The A2HBD has elevated expression in F. prausnitzii A2-165 and is crucial for the transformation of acetoacetyl-CoA to 3-hydroxybutyryl-CoA in the butyrate cycle. The monomeric structure of A2HBD consists of two domains, N-terminal and C-terminal, with cofactor binding occurring at the N-terminal domain, while the C-terminal domain facilitates dimerization. The A2HBD protein exists as a hexamer in solution.

To ascertain the binding mode of NAD+, we determined the 2.55Å resolution crystal structure of A2HBD in complex with NAD+ cofactor. In the structural analysis of the NAD+ complex derived from crystallography within the P21 space group, it was observed that all subunits comprising the hexameric assembly were found to bind to NAD+. By superposing the NAD-bound form of A2HBD with the apo-enzyme, we observed that the monomer structure of the NAD complex is similar to the apo-enzyme structure, displaying a root-mean-square deviation of 0.543Å. Like other NAD-dependent dehydrogenase enzymes, the NAD+ cofactor binds to the Rossmann fold domain without forming significant interactions with the C-terminal domain. Observing the binding mode of the NAD cofactor, adenine moiety of NAD cofactor is somewhat exposed to the surface of the enzyme, and the ribose and nicotinamide portion fitted into the deep cleft facing the acetyl group of the substrate. The phosphate moiety of the NAD cofactor resides within the G-x-G-x-x-G motif, composed of Gly7-Ala8-Gly9-Thr10-Met11-Gly12, situated between the initial β strand and the first α a helix within the Rossmann fold domain. The NAD cofactor is captured by the enzyme’s Thr10 and Met11 main-chain nitrogen atoms, establishing hydrogen bonds with the hydroxyl group of the phosphate moiety. Hydrogen bonding interactions involving Asp31, Glu90, Lys95, Asn115, and Ser117, along with hydrophobic interactions with Met11 and Phe138, contribute to the stabilization of the NAD cofactor’s two ribose rings and nicotinamide moiety. The hydrophobic pit accommodates the adenine moiety, fostering interactions with hydrophobic residues such as Ile6, Ile32, Ala88, Phe,89, Val94, and Thr98; thus contributing to the stabilization of the adenine phosphate. When comparing the catalytic triad′s conformational changes from the open to closed conformations, it becomes evident that in the NAD+ complex, characterized by an open conformation, the catalytic triad resides within a hydrogen bonding distance from each other, thereby contributing to the stabilization of these critical residues.

>[6x]MKIGVIGAGTMGQGIAKAFAQVEGNTVALCDIKQEWAENGLAKIKKGYEKLVAKGKIPQEKADAIVAAITPGLKENLCADCDLIVEAAFEDMKVKQTTFGELDKICKPECIFASNTSSLSITEIGKGLSRPLVGMHFFNPADRMKLIEVIAGCNTPAETVEKIKEISVAIGKNPVQVNEAAGFVVNRILIPMINEAAFIKMEGVSDIAGIDTAMKLGANHPMGPLELGDFIGLDICLAIMDVLYHETGDSKYRACPLIRKMVRGGNLGCKTGKGFYVYNADRTKTPVDQL>MTDEVVLLDFWPSPFGMRVRIALAEKGIEYEYKEEDLRNKSPLLLQMNPVHKKIPVLIHNGKPISESLIAVQYIEEVWNDRNPLLPSDPYQRAQARFWADYVDIKIHDLGKKIWTSKGEEKEAAKKEFIEALKLLEEQLGDKTYFGG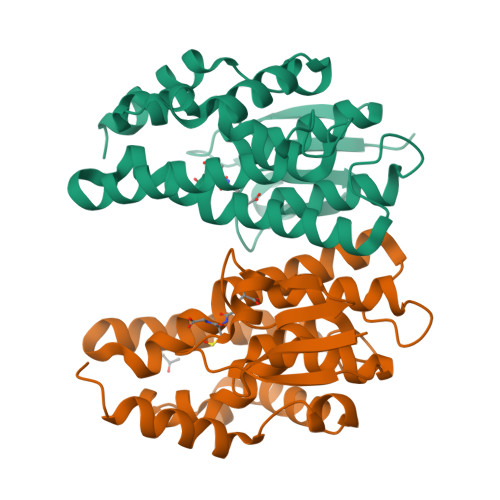DNIGFVDIALVPFYTWFKVYETFGSLNIENECPRFVAWAKRCLQKESVAKSLPDQHKVYEFVVEIRKKLVIE[2x]>DFVLDNEGN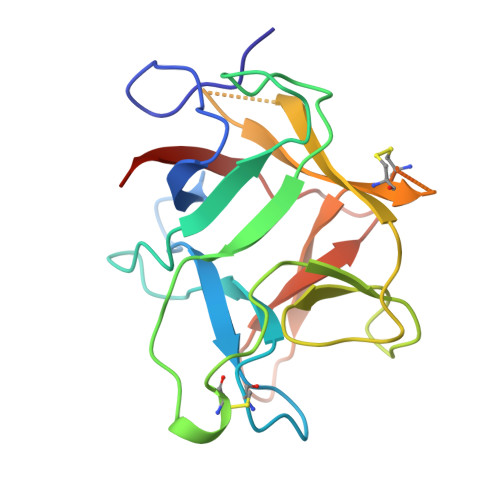PLENGGTYYILSDITAFGGIRAAPTGNERCPLTVVQSRNELDKGIGTIISSPYRIRFIAEGHPLSLKFDSFAVIMLCVGIPTEWSVVEDLPEGPAVKIGENKDAMDGWFRLERVSDDEFNNYKLVFCPQQAEDDKCGDIGISIDHDDGTRRLVVSKNKPLVVQFQKLDKESL[2x]>MLNYNAPTDGQKSSIDGANSDQMQTFFWLKKAIITARKEQYFMPLASVTNMPKHYGKTIKVYEYVPLLDDRNINDQGIDASGATIVNGNLYGSSK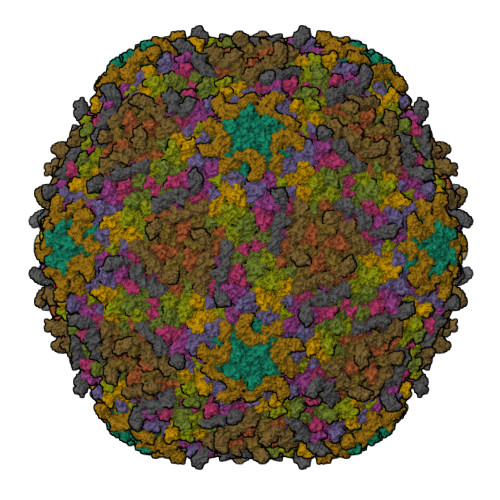DIGNITSKLPLLTENGGRVNRVGFTRIAREGSIHKFGFFYEFTQESIDFDSDDGLMEHLSRELMNGATQITEAVLQKDLLAAAGTVLYAGAATSDATITGEGSTPSVVSYKNLMRLDQILTENRTPTQTTIITGSRMIDTKVIGATRVMYVGSELVPELKAMKDLFGNKAFIETQHYADAGTIMNGEVGSIDKFRIIQVPEMLHWAGAGAQATGANPGYRTSMVSGQEHYDVYPMLVVGDDSFTSIGFQTDGKSLKFTVMTKMPGKETADRNDPYGETGFSSIKWYYGILVKRPERLALIKTVAPL[9x];>[3x]MPVLKVMFHKDTNVATVLDASGSLSDGSVEVGTFHHPDETYPDSVTIYHGVRDLLYKRSAKDPSQTASYPNNIINMQVISIDMKATPRLILGTALPRVISTIEGKDVTWHVDVAGGKAPLTYKWQFKANTVGAAFADIDSGENPTAKTATLINHAVTAESAGTYKVIVTDANGTTIESSSLLVVGVQEPPEVASIVAYPSPLALSVADDITDGKTVKFSSLPAGSLIGTLSIKTQPDSGKATAEISGNVLTVKPVAAGDTTVVVTNGTKEVTVTVNVTE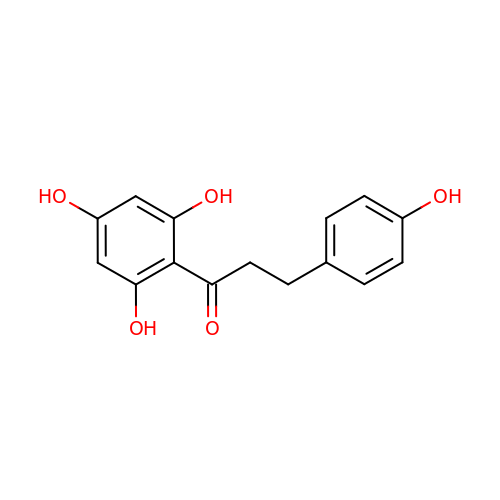3-(4-HYDROXYPHENYL)-1-(2,4,6-TRIHYDROXYPHENYL)PROPAN-1-ONE | C15 H14 O5 | VGEREEWJJVICBM-UHFFFAOYSA-N>AQ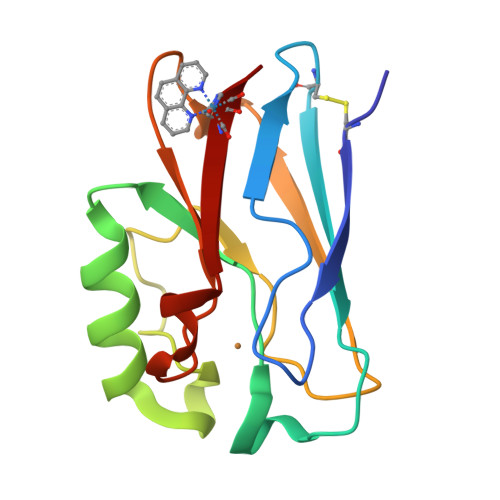CSVDIQGNDQMQFNTNAITVDKSCKQFTVNLSHPGNLPKNVMGHNWVLSTAADMQGVVTDGMASGLDKDYLKPDDSRVIAQTKLIGSGEKDSVTFDVSKLKEGEQYMFFCTFPGHSALMKGTLHLK[4x]>AESLPDLKIEKLDEGVYVHTSFEEVNGWGVVPKHGLVVLVNAEAYLIDTPFTAKDTEKLVTWFVERGYKIKGSISSHFHSESTGGIEWLNSRSIPTYASELTNELLKKDGKVQATNSFSGVNYWLVKNKIEVFYPGPGHTPDNVVVWLPERKILFGGCFIKPYGLGNLGDANIEAWPKSAKLLKS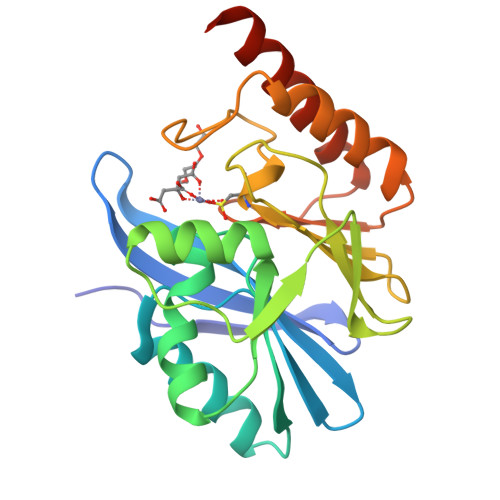KYGKAKLVVPSHSEVGDASLLKLTLEQAVKGLNESKKPSKPSN[4x]> ESKSPIIQNVLSYITEHFSEGMSLKTLGNDFHINAVYLGQLFQKEMGEHFTDYLNRYRVNYAKEELLQTKDN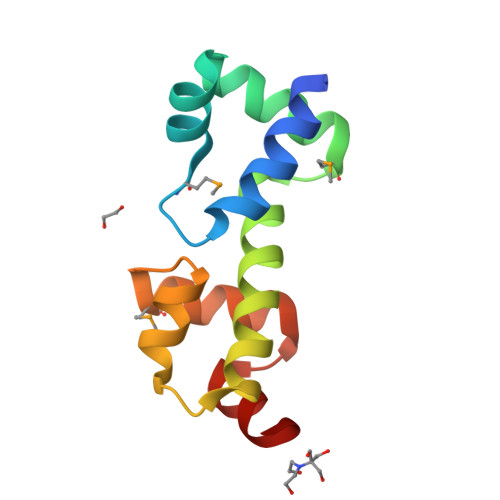LTIIAGKSGYTDMAYFYRQFKKHTGETPNRYRKIHQ>[2x]MTINYHELETSHGRIAVRESEGEGAPLLMIHGNSSSGAIFAPQLEGEIGKK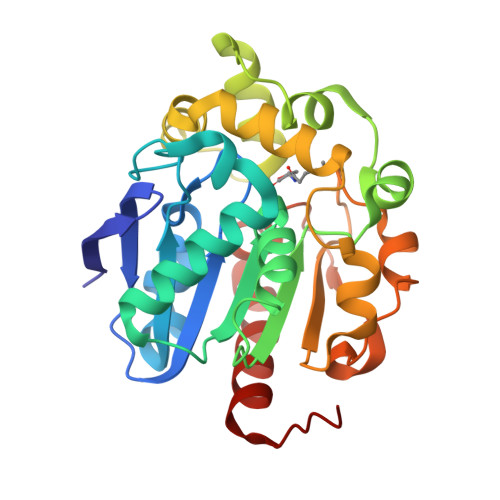WRVIAPDLPGHGKSTDAIDPDRSYSMEGYADAMTEVMQQLGIADAVVFGWGLGGHIGIEMIARYPEMRGLMITGTPPVAREEVGQGFKSGPDMALAGQEIFSERDVESYARSTCGEPFEASLLDIVARTDGRARRIMFEKFGSGTGGNQRDIVAEAQLPIAVVNGRDEPFVELDFVSKVKFGNLWEGKTHVIDNAGHAPFREAPAEFDAYLARFIRDCTQLEHHHHHH6-O-methylguanine | C6 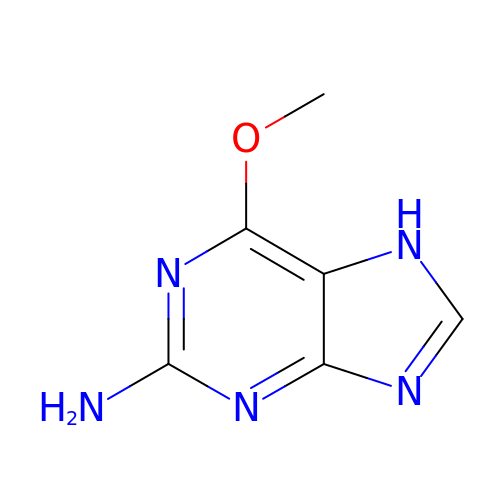H7 N5 O | BXJHWYVXLGLDMZ-UHFFFAOYSA-N>IKGGLFADIASHPWQAAIFAKHRRSPGERFLCGGILISSCWILSAAHCFQERFPPHHLTVILGRTYRVVPGEEEQKFEVEKYIVHKE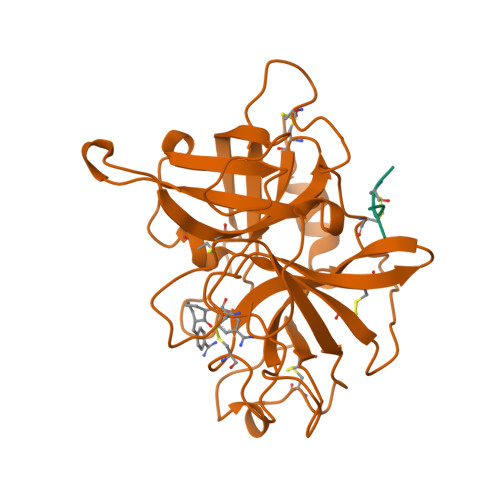FDDDTYDNDIALLQLKSDSSRCAQESSVVRTVCLPPADLQLPDWTECELSGYGKHEALSPFYSERLKEAHVRLYPSSRCTSQHLLNRTVTDNMLCAGDTRSGGPQANLHDACQGDSGGPLVCLNDGRMTLVGIISWGLGCGQKDVPGVYTKVTNYLDWIRDNMRP[2x];>[2x]TCGLRQY>[4x]MKIQMKTPLVELDGDEMTRVLWPLIKDKLLLPFIDLQTEYYDLGIEERDRTNDQITIDAAEAIKKYGVGVKNATITPNQDR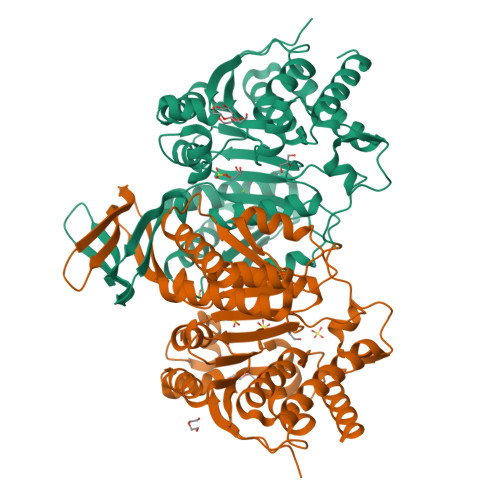VEEYGLKEQWKSPNATVRAMLDGTVFRKPIMVKNIKPSVRSWQKPIVVGRHAYGDFYKNAEIFAEAGGKLEIVVTDKNGKETRQTIMEVDEPAIVQGIHNTVASIGHFARACFEYSLDQKIDCWFATKDTISKQYDQRFKIIFEEIFAQEYKEKFAAAGIEYFYTLIDDVVARMMKTEGGMLWACKNYDGDVMSDMVASAFGSLAMMSSVLVSPYGYFEYEAAHGTVQRHYYQHLKGERTSTNPVALIYAWTGALRKRGELDGTPDLCAFCDSLEAITIECIESGYMTGDLARICEPAAIKVLDSIEFIDELGKRLQQLNK Wnt signalosome assembly relies on reversible head-to-tail polymerization by the N-terminal DIX domain of Dishevelled (Schwarz-Romond et al., 2007), which enables this hub to transduce Wnt signals to cytoplasmic effectors. In addition to DIX, Dishevelled has a PDZ domain (Post-synaptic density protein-95, Disc large tumor suppressor, Zonula occludens-1) and a DEP domain (Dishevelled, Egl-10, and Pleckstrin), separated by long flexible linkers peppered with phosphorylation sites, and also a binding motif for the AP2 clathrin adaptor (Yu et al., 2010). Here, we use structural analysis, as well as biophysical and cell-based assays, to show that the DEP domain of Dishevelled undergoes a conformational switch, from monomeric to swapped dimer, to trigger DIX-dependent polymerization and signaling to β-catenin. This occurs in two steps: binding of monomeric DEP to Frizzled followed by DEP domain swapping triggered by its high local concentration upon Wnt-induced recruitment into clathrin-coated pits.

Purifying lipoyl-tagged DEP (Lip-DEP416–511) by size exclusion chromatography (SEC), we observed two main peaks, corresponding to monomers and dimers (discussed later), in addition to a higher mass species. Thus, we crystallized the monomeric and dimeric fractions and determined three structures at 1.84–2.06 Å resolution. Remarkably, each structure exhibits a swapped dimer, regardless of the crystal form: namely, molecule A (turquoise) donates H1 to the H2–H3 core of molecule B (light turquoise) by extending loop 1, and vice versa. Thus, two DEP cores are connected by an extended β sheet, composed of two antiparallel β strands (each made up by a β1β2 tandem) that interact with each other through backbone atoms of residues 442–447. This dimer-specific interface is based on six new hydrogen bonds, which may bias the equilibrium toward the domain-swapped configuration. Interestingly, the solvent-exposed “underside” of the connecting β sheet presents a hydrophobic patch, made up of a triad of hydrophobic amino acids (M443, L445, and I447) located at the DEP finger tip of the monomer. In each crystal, two DEP dimers associate with each other through this hydrophobic patch, thus linking four DEP cores into a cross-shaped tetramer. Presumably, the high protein concentration in the crystallization drops favored the tetramerization of DEP. The first condition is met by the clathrin-coated pits in which multiple Dishevelled molecules are juxtaposed, potentially reaching a very high local concentration which could be sufficient to induce DEP dimerization. Thus, they mimic the conditions during DEP crystallization, which inexorably induced domain swapping.

>[4x]SSGLSVHTDMASVTKAMAAPESGLEVRDRMWLKITIPNAFLGSDVVDWLYHHVEGFPERREARKYASGLLKAGLIRHTVNKITFSEQCYYVFGDLSG>MFVNKQFNYKDPVNGVDIAYIKIPNAGQMQPVKAFKIHNKIWVIPERDTFTNPEEGDLNPPPEAKQVPVSYYDSTYLSTDNEKDNYLKGVTKLFERIYSTDLGRMLLTSIVRGIPFWGGSTIDTELKVIDTNCINVIQPDGSYRSEELNLVIIGPSADIIQFECKSFGHDVLNLTRNGYGSTQYIRFSPDFTFGFEESLEVDTNPLLGAGKFATDPAVTLAHELIHAEHRLYGIAINPNRVFKVNTNAYYEMSGLEVSFEELRTF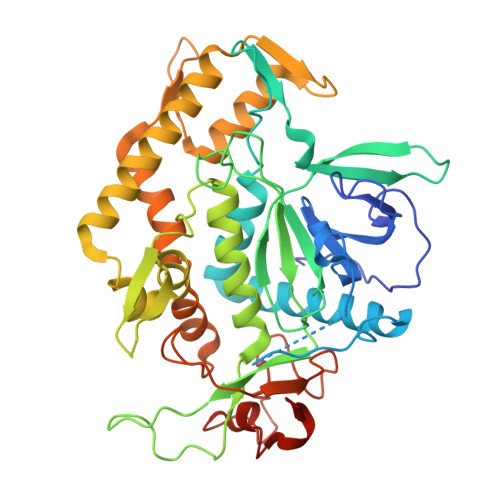GGHDAKFIDSLQENEFRLYYYNKFKDVASTLNKAKSIIGTTASLQYMKNVFKEKYLLSEDTSGKFSVDKLKFDKLYKMLTEIYTEDNFVNFFKVINRKTYLNFDKAVFRINIVPDENYTIKDGFNLKGANLSTNFNGQNTEINSRNFTRLKNFTGLFEFY[2x]>SQKSWIESTLTKRECVYIIPSSKDPHRCLPGCQICQQLVRCFCGRLVKQHACFTASLAMKYSDVKLGEHFNQAIEEWSVEKHTEQSPTDAYGVINFQGGSHSYRAKYVRLSYDTKPEIILQLLLKEWQMELPKLVISVHGGMQKFELHPRIKQLLGKGLIKAAVTTGAWILTGGVNTGVAKHVGDALKEHASRSSRKICTIGIAPWGVIENRNDLVGRDVVAPYQTLLNPLSKLNVLNNLHSHFILVDDGTVGKYGAEVRLRRELEKTINQQRIHARIGQGVPVVALIFEGGPNVILTVLEYLQESPPVPVVVCEGTGRAADLLAYIHKQTEEGGNLPDAAEPDIISTIKKTFNFGQSEAVHLFQTMMECMKKKELITVFHIGSEDHQDIDVAILTALLKGTNASAFDQLILTLAWDRVDIAKNHVFVYGQQWLVGSLEQAMLDALVMDRVSFVKLLIENGVSMHKFLTIPRLEELYNTKQGPTNPMLFHLIRDVKQGNLPPGYKITLIDIGLVIEYLMGGTYRCTYTRKRFRLIYNSLGGNNRRSGRNTSSSTPQLRKSHETFGNRADKKEKMRHNHFIKTAQPYRPKMDASMEEGKKKRTKDEIVDIDDPETKRFPYPLNELLIWACLMKRQVMARFLWQHGEESMAKALVACKIYRSMAYEAKQSDLVDDTSEELKQYSNDFGQLAVELLEQSFRQDETMAMKLLTYELKNWSNSTCLKLAVSSRLRPFVAHTCTQMLLSDMWMGRLNMRKNSWYKVILSILVPPAILMLEYKTKAEMSHIPQSQDAHQMTMEDSENNFHNITEEIPMEVFKEVKILDSSDGKNEMEIHIKSKKLPITRKFYAFYHAPIVKFWFNTLAYLGFLMLYTFVVLVKMEQLPSVQEWIVIAYIFTYAIEKVREVFMSEAGKISQKIKVWFSDYFNVSDTIAIISFFVGFGLRFGAKWNYINAYDNHVFVAGRLIYCLNIIFWYVRLLDFLAVNQQAGPYVMMIGKMVANMFYIVVIMALVLLSFGVPRKAILYPHEEPSWSLAKDIVFHPYWMIFGEVYAYEIDVCANDSTLPTICGPGTWLTPFLQAVYLFVQYIIMVNLLIAFFNNVYLQVKAISNIVWKYQRYHFIMAYHEKPVLPPPLIILSHIVSLFCCVCKRRKKDKTSDGPKLFLTEEDQKKLHDFEEQCVEMYF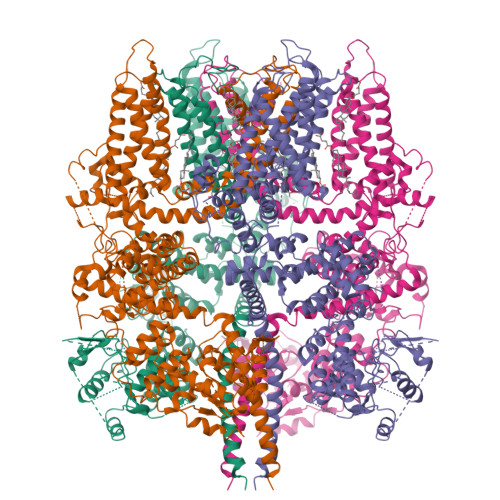DEKDDKFNSGSEERIRVTFERVEQMSIQIKEVGDRVNYIKRSLQSLDS[4x]5-[(2,3-dichlorophenoxy)methyl]furan-2-carboxylic acid | C12 H8 Cl2 O4 | 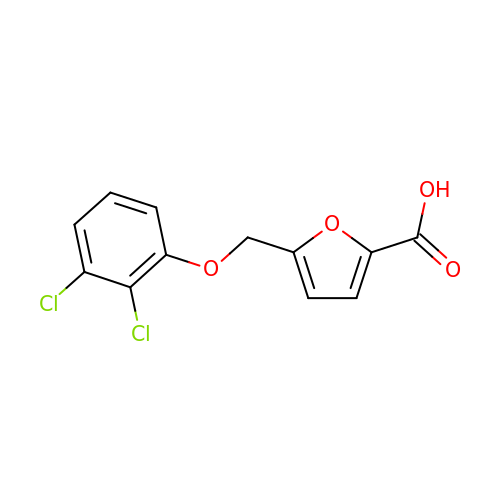DGUXQMFHNWGUES-UHFFFAOYSA-N> GGGRMEGESTLGVLSGFVLGALTFHHLNTDSDTEGFLLGEMKGEAKNSITDSQMDNVKVVYTIDIQKYIPCYRLFSFYNSLGEVNEHALKKVLSNVRKTVVGWYKFRRHSDQIMTFREQLLHRNLQTHLSSPELVFLLLTPSITTESCSTHCLEHALYKPQRGLFHRVPLVVTNLGMSDQLGYKTEPASCTSTVFSRAVRTHSSQFFNEDGSLKEVHKINEMYAAVQEELKSICQKVEQSEREVEKLLMDVNQLKEVRRTQQARA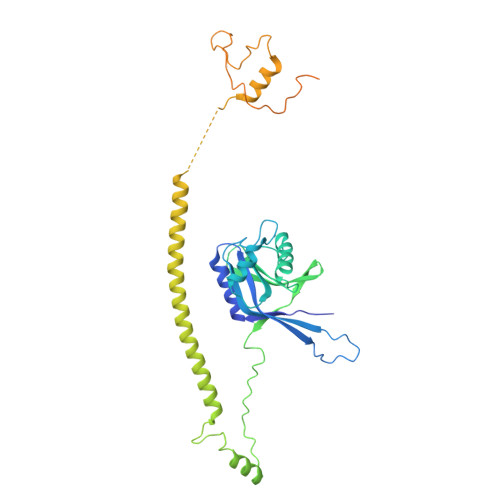TGAGEKNVQRNPQENILLCQALRTFFPESEVLHSCVISLKNRHISPSGCNVNHHVDVVDQLTLMVEYVYSPEASPVPTAQLRKRKALDTHDQGSVKRPRLLETESRPSVAASRSRHQDKASSSSLDIDIEMGSPEDDADYPRSPTF> SGAKPGKKTRGRVKIKMEFIDNKLRRYTTFSKRKTGIMKKAYELSTLTGTQVLLLVASETGHVYTFATRKLQPMITSETGKALIQTC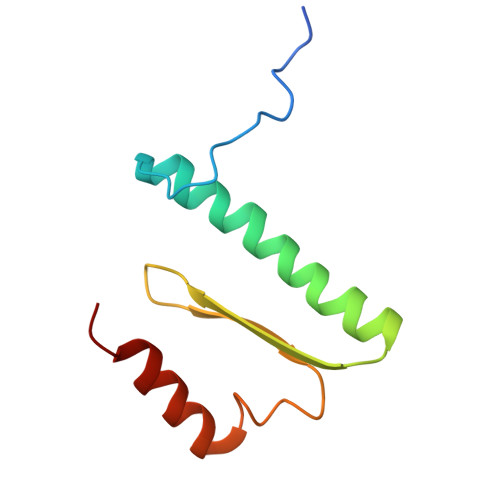LNSPD> HTLKTANSYTDVTVSNSTKKAIRESN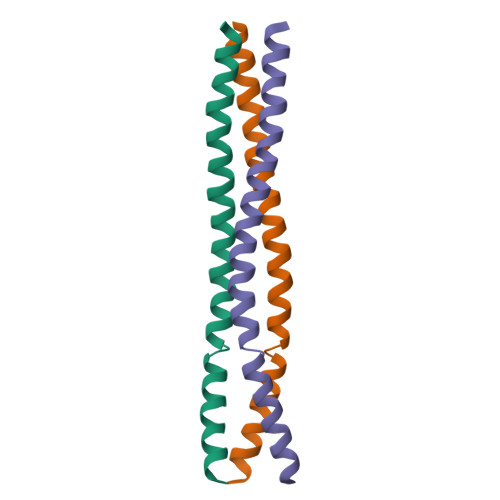QYTDHKFHQLDNRLDKLDTRLLKLLASSAALNSLL> G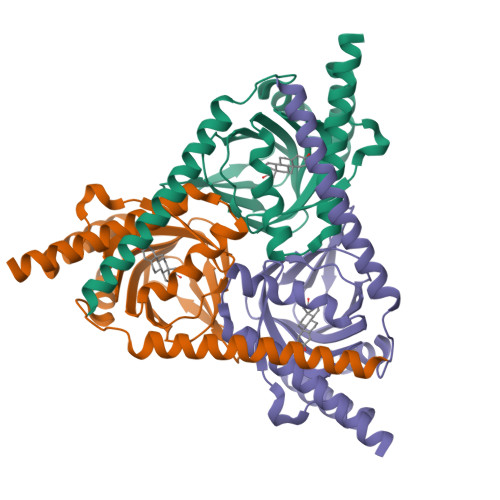GGGRSVDTMALWLGLRAVLVVAGLAVLLQLIRGWLSSKSYVFNREEIARLAKEHSGLDYEVAFSKIIVELRKKHPGHILQDEDLQWVFVNAGGWMGSMCLLHASLTEYVLLFGTAVDTGGHSGRYWAEISDTILSGTFRQWKEGTTKSEIFYPGDTIVHEVGEATSVQWSSGTWMVEYGRGFIPSTLAFALADTIFSTQDFLTLFYTVKVYSKALLLEASTHLSQLGFFAAA(S)-2-[(R)-3-AMINO-4-(2-FLUORO-PHENYL)-BUTYRYL]-1,2,3,4-TETRAHYDRO-ISOQUINOLINE-3-CARBOXYLIC ACID AMIDE | C20 H22 F N3 O2 | 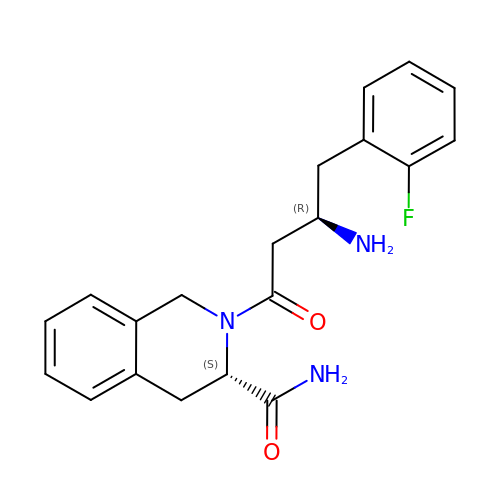OEVYDSSAPNIURZ-AEFFLSMTSA-N>[2x]MWVYRLKGTLEALDPILPGLFDGGARGLWEREGEVWAFFPAPVDLPYEGVWEEVGDEDWLEAWRRDLKPALAPPFVVLAPWHTWEGAEIPLVIEPGMAF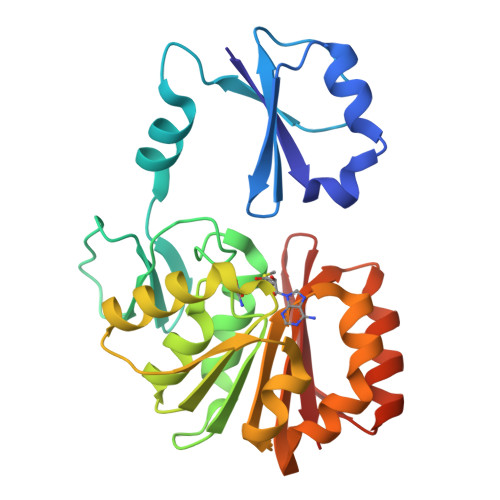GTGHHETTRLALKALARHLRPGDKVLDLGTGSGVLAIAAEKLGGKALGVDIDPMVLPQAEANAKRNGVRPRFLEGSLEAALPFGPFDLLVANLYAELHAALAPRYREALVPGGRALLTGILKDRAPLVREAMAGAGFRPLEEAAEGEWVLLAYGR One enzyme, triosephosphate isomerase (TIM; EC 5.3.1.1), is of particular interest as an anthelmintic target. TIM catalyzes the isomerization of glyceraldehyde-3-phosphate and dihydroxyacetone phosphate in the fifth step of the glycolytic pathway. Structurally, most of the known TIMs are homodimers, each monomer consisting of eight parallel β-strands surrounded by eight α-helices that, together, form a typical “TIM barrel” fold. Because TIM is active only in its dimeric form, small molecules that engage the interface may interfere with proper enzyme function.

To elucidate the molecular basis of FhTIM inhibition, we obtained the crystal structure of FhTIM at 1.9 Å resolution. The asymmetric unit displays three FhTIM dimers. Each protomer shows a typical (β/α)8 TIM-barrel fold. The catalytic pocket of each protomer in the FhTIM structure is occupied by a sulfate molecule (SO42−), likely from the crystallization buffer. The β/α loop 6 (residues 168–180 of FhTIM) is known to open and close when accommodating the substrate in triosephosphate isomerases. Here, the loops are in the close conformation in all of the protomers of FhTIM. Interestingly, the SO42− ion is located in the same position as the phosphate group of the substrates (glyceraldehyde 3 P) in the P. falciparum (Pf TIM) or S. aureus TIM structures (PDB ID: 1LYX15 and 3UWU24, respectively) through similar interactions. Indeed, the three unbound oxygen atoms of the O4 tetrahedron in the triose phosphate moiety of Pf TIM interact with the main chain nitrogen of residues G175, S211, G236 and G237, as do 3 out of 4 oxygen atoms of the FhTIM SO42−. The remaining oxygen of the SO42− present in the FhTIM structure (and spatially corresponding to the oxygen atom linking the phosphate to the sugar in the natural substrate) is coordinated by a water molecule roughly located at the position of the distal carbon of the substrate analog in Pf TIM. Attempts to understand the mechanism of interaction between the inhibitors and TIM via crystallization did not yield ligand-bound structures.

>ASNRKFFVGGNWKMNGSKESNQKLLKTLSDAKPDANTEILVAVPFVYLKDVREHLDKRFHVAAQNCYKVASGAFTGEISPAMIRDCGCEWVILGHSERRHIFGESDELIGEKVNHALTCGLKVVPCIGEKLDEREAGKTEQVCFRQLDAIKKGIPKAEDWSRVVIAYEPVWAIGTGKTASPEQAQEVHHAVRQWLEKNVSQAVASSLRITYGGSVTAANCKELAKKPDVDGFLVGGASLKPEFVDICNAN[6x]>NRLSVKLPGLDLKNPIIPASGCFGFGEEYAKYYDLNKLGSIMVKATTLHPRFGNPTPRVAETASGMLNADGLQNPGLEVIMAEKLPWLNENFPDLPIIANVAGSEEDDYVAVCAKIGDAPNVKVIELNISCPNVKHGGQAFGTDPDVAAALVKACKAVSKVPLYVKLSPNVTDIVPIAKAVEAAGADGLTMINTLMGVRFDLKTRKPVLANITGGLSGPAIKPVALKLIHQVAQVVDIPIIGMGGVESAQDVLEMYMAGASAVAVGTANFADPFVCPKIIEKLPEVMDQYGIDSLENLIQEVKNSK[2x];>MPKLQEMMTIVSQREVASNIFE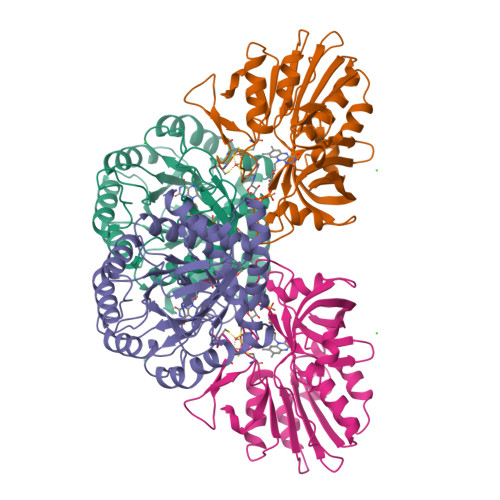MVLKGELVEEMDLPGQFLHLAVPNASMLLRRPISISSWDKVAKTCTILYRIGDETSGTYEISKLQSGAKIDVMGPLGNGFPVDEVVSTDKILIVGGGIGVPPLYELAKQLEEKNCQMTILLGFASEKVKILEKEFAELKNVSLKIATDDGSYGTKGHVGMLMEEIDFEVDALYTCGAPAMLKAVAKKYEQLERLYISMESRMACGIGACYACVEHDKEDENHALKVCEDGPVFLGKQLLL[2x]N~5~-(N-ethoxycarbamimidoyl)-L-ornithine | C8 H18 N4 O3 | 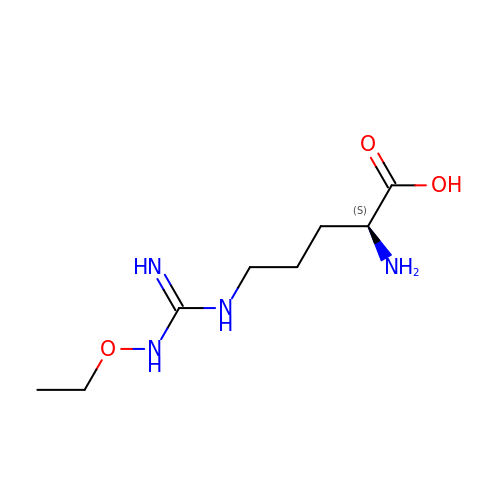RVVPNRVWAPOQMA-LURJTMIESA-N> GDSIEDKNARVIELIAAYRNRGHLMADIDPLRLDNTRFRSHPDLDVNSHGLTLWDLDREFKVDGFAGVQRKKLRDILSVLRDAYCRHVGVEYTHILEPEQQRWIQERVETKHDKPTVAEQKYILSKLNAAEAFETFLQTKYVGQKRFSLEGAETVIPMMDAVIDQCAEHGLDEVVIAMPHRGRLNVLANIVGKPYSQIFSEFEGNLNPSQAHGSGDVKYHLGATGTYIQMFGDNDIEVSLTANPSHLEAVDPVL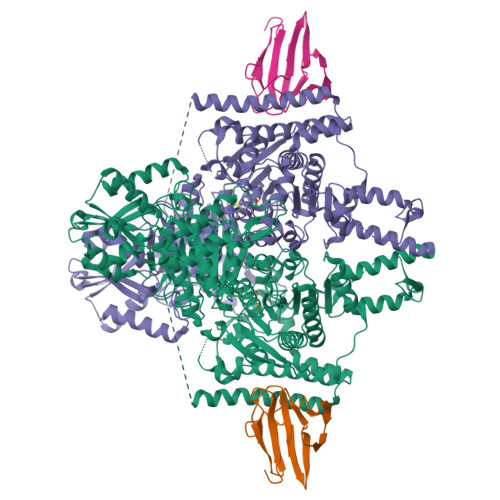EGLVRAKQDLLDTGEEGSDNRFSVVPLMLHGDAAFAGQGVVAETLNLALLRGYRTGGTIHIVVNNQIGFTTAPTDSRSSEYCTDVAKMIGAPIFHVNGDDPEACAWVARLAVDFRQAFKKDVVIDMLCYRRRGHNEGDDPSMTQPYMYDVIDTKRGSRKAYTEALIGRGDISMKEAEDALRDYQGQLERVFNEVRELEKHEIEPSESVEADQQIPSKLATAVDKAMLQRIGDAHLALPEGFTVHPRVRPVLEKRREMAYEGRIDWAFAELLALGSLIAEGKLVRLSGQDTQRGTFTQRHAVIVDRKTGEEFTPLQLLATNPDGTPTGGKFLVYNSALSEFAAVGFEYGYSVGNPDAMVLWEAQFGDFVNGAQSIIDEFISSGEAKWGQLSDVVLLLPHGHEGQGPDHTSGRIERFLQLWAEGSMTIAMPSTPANYFHLLRRHGKDGIQRPLIVFTPKSMLRNKAAVSDIRDFTESKFRSVLEEPMYTDGEGDRNKVTRLLLTSGKIYYELAARKAKENREDVAIVRIEQLAPLPRRRLAETLDRYPNVKEKFWVQEEPANQGAWPSFGLTLPEILPDHFTGLKRISRRAMSAPSSGSSKVHAVEQQEILDTAFG;> GSGVEGLPSGSALLVVKRGPNAGSRFLLDQPTTSAGRHPDSDIFLDDVTVSRRHAEFRLEGGEFQVVDVGSLNGTYVNREPVDSAVLANGDEVQIGKFRLVFLTGPKSDDSGSNA>SNAMLRRLFKKKYVCVRQYDLTDCGAACLSSIAQYYGLKMSLAKIREMTGTDTQGTNAYGLIHAAKQLGFSAKGVKASKEDLLKDFRLPAIANVIVDNRLAHFVVIYSIKNRIITVADPGKGIVRYSMDDFCSIWTGGLVLLEPGEAFQKGDYTQNMMVKFAGFLKPLKKTVLCIFLASLLYTALGIAGSFYIKFLFDDLIKFEKLNDLHIISAGFAVIFLLQIFLNYYRSILVTKLGMSIDKSIMMEYYSHVLKLPMNFFNSRKVGEIISRFMDASKIRQAISGATLTIMIDTIMAVIGGILLYIQNSSLFFISFIIILLYGIIVTVFNKPIQNANRQIMEDNAKLTSALVESVKGIETIKSFGAEEQTEKSTRDKIETVMKSSFKEGMLYINLSSLTGIVAGLGGIVILWAGAYNVIKGNMSGGQLLAFNALLAYFLTPVKNLIDLQPLIQTAVVASNRLGEILELATEKELREDSDDFVISLKGDIEFRNVDFRYGLRKP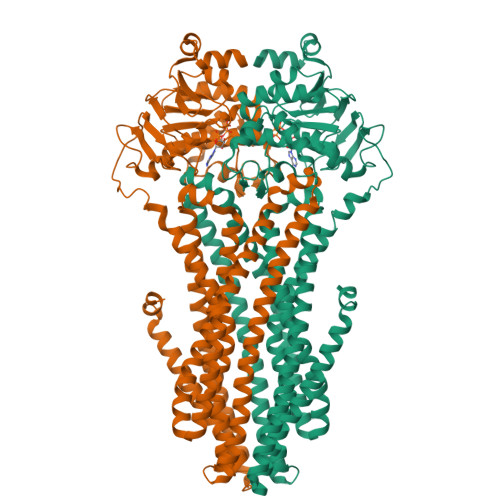VLKNINLTIPKGKTVAIVGESGSGKTTLAKLLMNFYSPEKGDILINGHSIKNISLELIRKKIAFVSQDVFIFSGTVKENLCLGNENVDMDEIIKAAKMANAHDFIEKLPLKYDTFLNESGANLSEGQKQRLAIARALLKKPDILILDQATSNLDSITENHIKDAIYGLEDDVTVIIIAHRLSTIVNCDKIYLLKDGEIVESGSHTELIALKGCYFKMWKQTENTLAS[2x]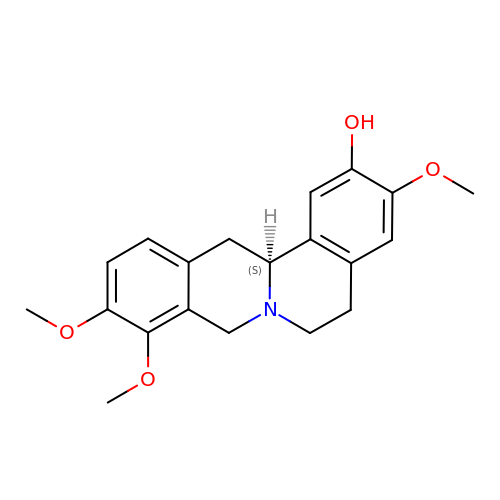Tetrahydrocolumbamine | C20 H23 N O4 | KDFKJOFJHSVROC-INIZCTEOSA-N4-amino-2-[4-(tert-butylsulfamoyl)phenyl]-N-methylthieno[3,2-c]pyridine-7-carboxamide | C19 H22 N4 O3 S2 | 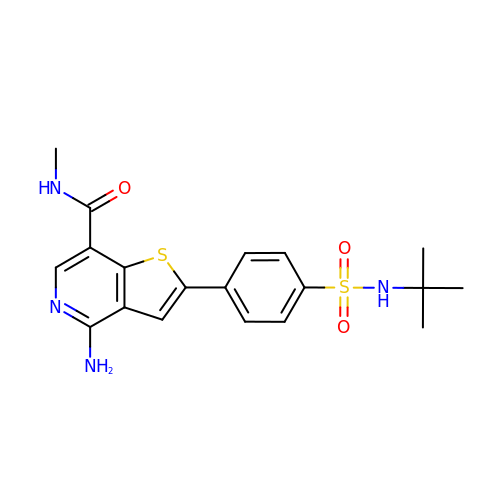FVVCSMCEMMLEGG-UHFFFAOYSA-N> MSSFTHFNEQGRAKMVDITHKEDTVRVAVAQTSVTVSREIYEKMTSNAIEKGDVLAVAQVAGVMAAKKTADLIPMCHPLMLKGVDIAFAWENDGEAHKLVITATVKTKGSTGVEMEALTAASVCALT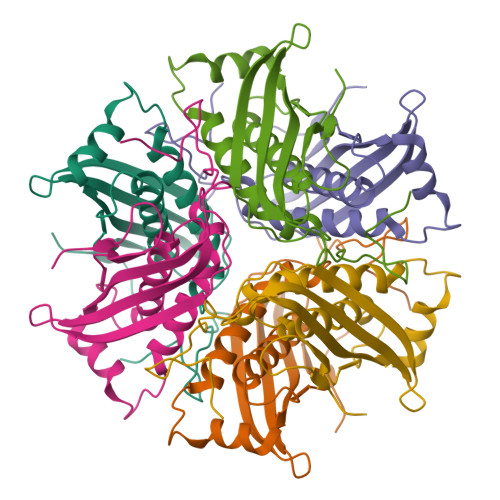VYDMCKALDKGMVIGPTYLVEKTGGKSGHYRRKTD> GPLGSGNIFIKNLDKSIDNKALYDTFSAFGNILSCKVVCDENG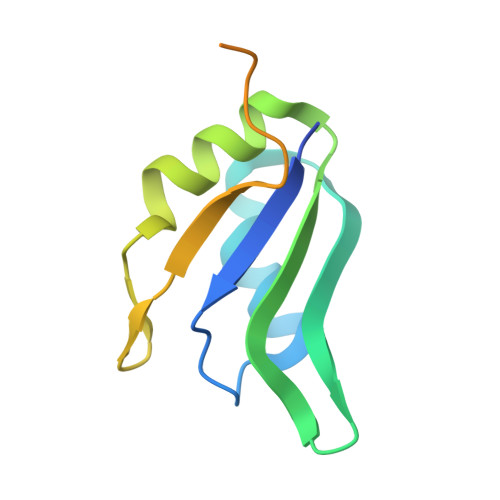SKGYGFVHFETQEAAERAIEKMNGMLLNDRKVFVGRFKSRKEREAELGARAKEFTNVYIKNFGPGSTRAAAS> MLSKALQRGIARAFSTTAKKEAPKTVKANGQVSQVIGAVVDVQFEGELPQILNALEVQGTQHRLVLEVAQHLGDSRVRTIAMDSTEGLVRGQPVVDTGLPISVPVGPGTLGRIMNVIGEPIDQRGPIKAAKLYPIHRDAPSFTDQATSAEILVTGIKVVDLLAPYARGGKIGLFGGAGVGKTVLIQELINNVAKHHGGYSVFAGVGERTREGNDLYHEMMDSKVISVKEGESRCALIFGQMNEPPGARARVGLTGLTVAEYFRDEEGKDVLLFVDNIFRFTQACSEVSALLGRIPSAVGYQPTLATDLGALQERITTT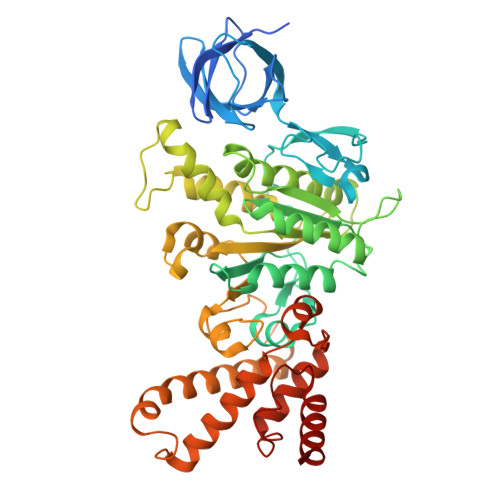QKGSITSVQAIYVPADDLTDPAPATTFAHLDATTVLNRGLTELGIYPAVDPLDSTSRMLDPITIGEEHYTVARGVQKLLQDYKSLQDIIAILGVDDLSEEDKLVVARARKVQKFLSQPFFMSEVFSGIPGRFVNLKQNIASFKALLEGAGDEYPESCFYMKGDLEESLAAGRADALKSK>[6x]MGSSHHHHHHSQDPKPRVLVLTGAGISAESGIRTFRAADGLWEEHRVEDVGTPEGFDRDPELVQAFYNARRRQLQQPEIQPNAAHLALAKLQDALGDRFLLVTQNCDNLHERAGNTNVIHMHGELLKVRCSQSGQALDWTGDVTPEDKCHCCQFPAPLRPHVVWFGEMPLGMDEIYMALSMADIFIAIGTSGHVYPAAGFVHEAKLHGAHTVELNLEPSQV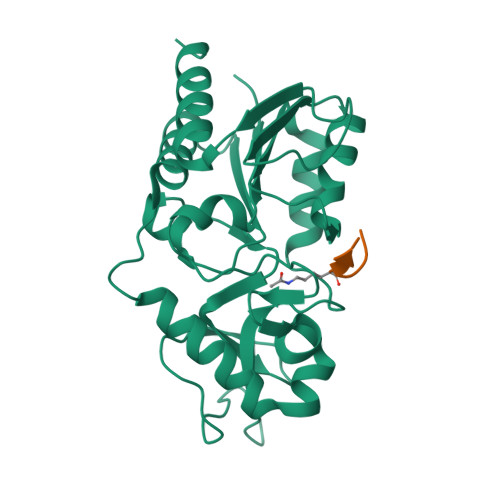GNEFAEKYYGPASQVVPEFVEKLLKGLKAGSIA;>KGGAKRHRKIL[6x]> METTVLVTFEQRLTTGDVGKLSRLIGAVIPIPYRHHLLGSSQVGLDAVVKDKTRDYSRMRARMREMTLTIMRRVEGNQMILGVPTHGQCYTIRNTGPVSWEKGDVLTTLPPVFSGEVTGLVSVSDWDLVLPWIVPMALATEINQRMMMLALLSLDRSHEEVRAATAQLRVVRYRDATLTLPEITIDDTVLIDMRNVCISLSMIANLSSEVTLAYVRKLA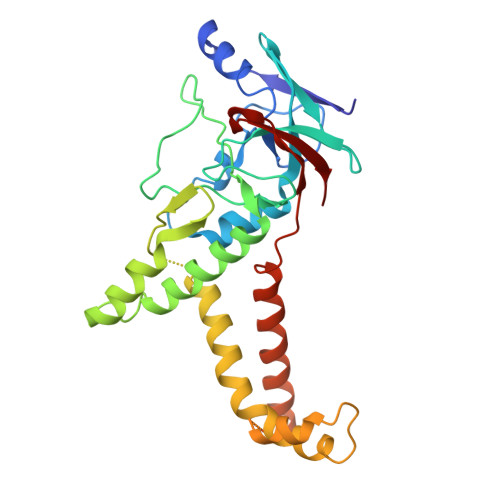LEDSNMLLMKCQEILGRRMPQVGVGAGSSGDRNDPPARSRTNYNITPTEELNKLTALFVMIRQITDVISEQPAFLVCDVSPDDKSALCIYKG> MSRKRSTKPKPAAKIALKKENDQFLEALKLYEGKQYKKSLKLLDAILKKDGSHVDSLALKGLDLYSVGEKDDAASYVANAIRKIEGASASPICCHVLGIYMRNTKEYKESIKWFTAALNNGSTNKQIYRDLATLQSQIGDFKNALVSRKKY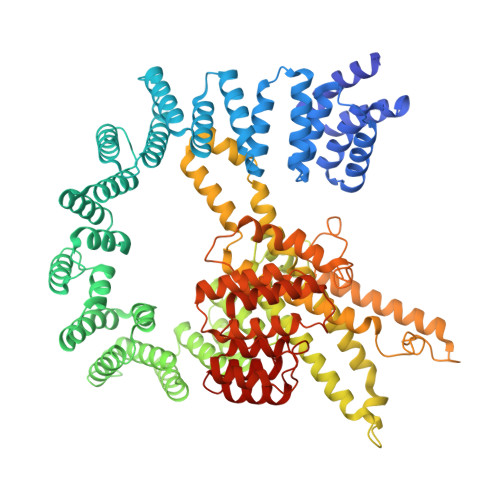WEAFLGYRANWTSLAVAQDVNGERQQAINTLSQFEKLAEGKISDSEKYEHSECLMYKNDIMYKAASDNQDKLQNVLKHLNDIEPCVFDKFGLLERKATIYMKLGQLKDASIVYRTLIKRNPDNFKYYKLLEVSLGIQGDNKLKKALYGKLEQFYPRCEPPKFIPLTFLQDKEELSKKLREYVLPQLERGVPATFSNVKPLYQRRKSKVSPLLEKIVLDYLSGLDPTQDPIPFIWTNYYLSQHFLFLKDFPKAQEYIDAALDHTPTLVEFYILKARILKHLGLMDTAAGILEEGRQLDLQDRFINCKTVKYFLRANNIDKAVEVASLFTKNDDSVNGIKDLHLVEASWFIVEQAEAYYRLYLDRKKKLDDLASLKKEVESDKSEQIANDIKENQWLVRKYKGLALKRFNAIPKFYKQFEDDQLDFHSYCMRKGTPRAYLEMLEWGKALYTKPMYVRAMKEASKLYFQMHDDRLKRKSDSLDENSDEIQNNGQNSSSQKKKAKKEAAAMNKRKETEAKSVAAYPSDQDNDVFGEKLIETSTPMEDFATEFYNNYSMQVREDERDYILDFEFNYRIGKLALCFASLNKFAKRFGTTSGLFGSMAIVLLHATRNDTPFDPILKKVVTKSLEKEYSENFPLNEISNNSFDWLNFYQEKFGKNDINGLLFLYRYRDDVPIGSSNLKEMIISSLSPLEPHSQNEILQYYL>[2x]GSHMSRLLEDFRNQRYPNLQLRDLA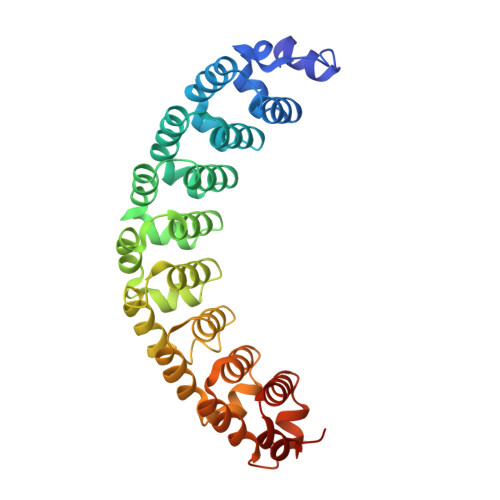NHIVEFSQDQHGSRFIQQKLERATAAEKQMVFSEILAAAYSLMTDVFGNYVIQKFFEFGTPEQKNTLGMQVKGHVLQLALQMYGCRVIQKALESISPEQQQEIVHELDGHVLKCVKDQNGNHVVQKCIECVDPVALQFIINAFKGQVYSLSTHPYGCRVIQRILEHCTAEQTTPILDELHEHTEQLIQDQYGNYVIQHVLEHGKQEDKSILINSVRGKVLVLSQHKFASNVVEKCVTHATRGERTGLIDEVCTFNDNALHVMMKDQYANYVVQKMIDVSEPTQLKKLMTKIRKNMAAL> MADFLNFPRQMLPFSKKTKQWRKDCLLWANQKTFFNYSLVRKSVIHKKINYDLLNGRLHMSDLELVLNPDGIKAAYIPDRLQHYPIMNSKLNVLRGEESKRVFDFKVVVTNPNAISEIEDNKKNELLQRLQEMITDTSISEDEYNIKLEKLNDYYTYEWQDIREVRANELLNHYIKEYDIPLIFNNGFMDAMTCGEEIY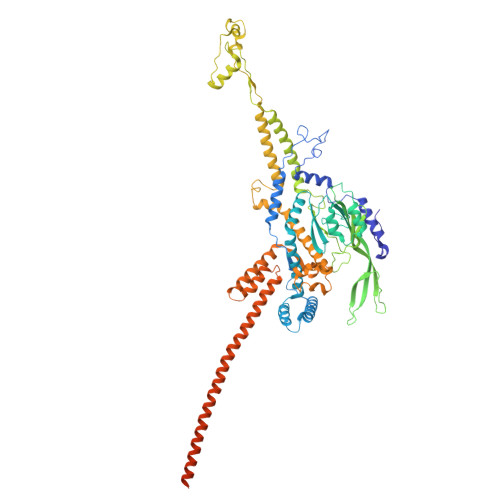QCDIVGGEPVIERVNPLKIRIFKSGYSNKVEDADMIILEDYWSPGRVIDTYYDVLSPKDIKYIETMPDYIGQGAVDQMDNIDERYGFVNQNMIGDEITVRDGTYFFDPANLFTEGIANSLLPYDLAGNLRVLRLYWKSKRKILKVKSYDPETGEEEWNFYPENYVVNKEAGEEVQSFWVNEAWEGTMIGNEIFVNMRPRLIQYNRLNNPSRCHFGIVGSIYNLNDSRPFSLVDMMKPYNYLYDAIHDRLNKAIASNWGSILELDLSKVPKGWDVGKWMYYARVNHIAVIDSFKEGTIGASTGKLAGALNNAGKGMIETNIGNYIQQQINLLEFIKMEMADVAGISKQREGQISQRETVGGVERATLQSSHITEWLFTIHDDVKKRALECFLETAKVALKGRNKKFQYILSDTSTRVMEIDGDEFAEADYGLVVDNSNGTQELQQKLDTLAQAALQTQTLSFSTITKLYTSSSLAEKQRLIEKDEKQIRERQAQAQKEQLEAQQQIAAMQQQQKEAELLQKEEANIRDNQTKIIIAQIQSEGGPDEEDGIMIDDYSPEAKANLAEKIREFDEKLKLDKDKLKLDKKKAETDASIKRQALRKKSSTTNK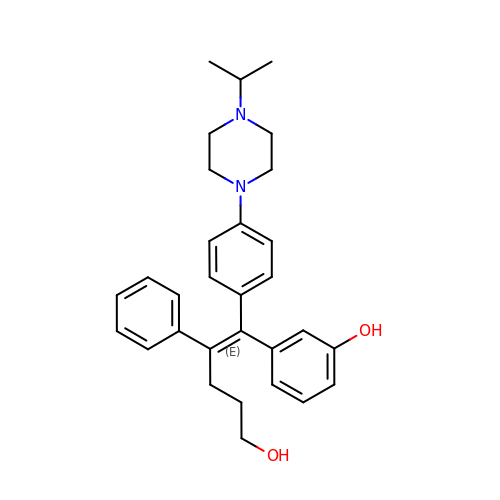3-[(~{E})-5-oxidanyl-2-phenyl-1-[4-(4-propan-2-ylpiperazin-1-yl)phenyl]pent-1-enyl]phenol | C30 H36 N2 O2 | MVDJTCFLEZIJEJ-QVIHXGFCSA-N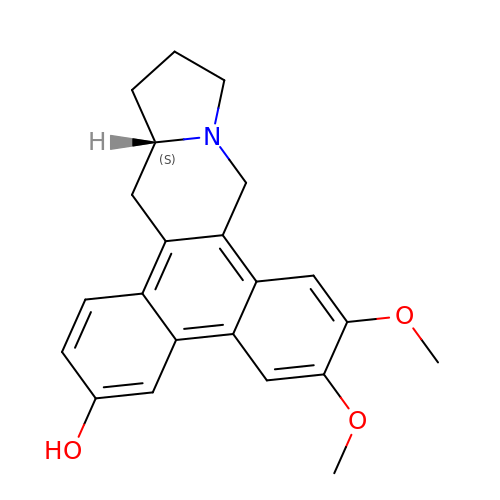(13~{a}~{S})-6,7-dimethoxy-9,11,12,13,13~{a},14-hexahydrophenanthro[9,10-f]indolizin-3-ol | C22 H23 N O3 | DSYIHAGYTDJTNX-ZDUSSCGKSA-N>MADDQGCIEEQGVEDSANEDSVDAKPDRSSFVPSLFSKKKKNVTMRSIKTTRDRVPTYQYNMNFEKLGKCIIINNKNFDKVTGMGVRNGTDKDAEALFKCFRSLGFDVIVYNDCSCAKMQDLLKKASEEDHTNAACFACILLSHGEENVIYGKDGVTPIKDLTAHFRGDRCKTLLEKPKLFFIQACRGTELDDGIQAD[2x];>SGPINDTDANPRYKIPVEADFLFAYSTVPGYYSWRSPGRGSWFVQALCSILEEHGKDLEIMQILTRVNDRVARHFESQSDDPHFHEKKQI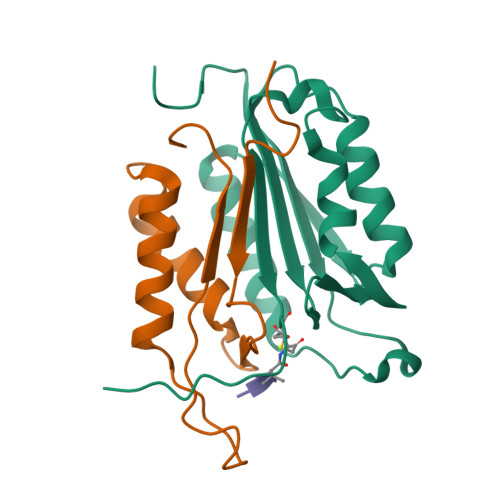PCVVSMLTKELYFSQLEHHHHHH[2x]> IMRHLPYFCRGQVVRGFGRGSKQLGIPTANFPEQVVDNLPADISTGIYYGWASVGSGDVHKMVVSIGWNPYYKN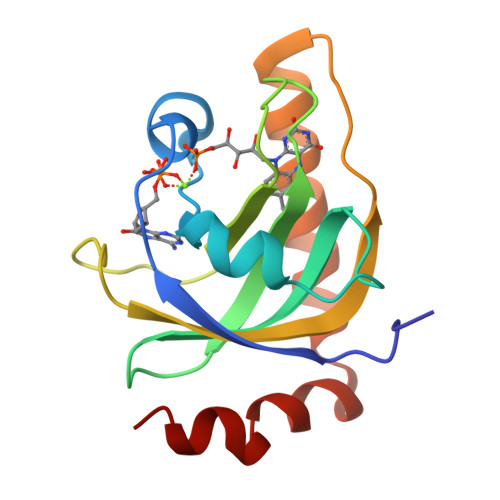TKKSMETHIMHTFKEDFYGEILNVAIVGYLRPEKNFDSLESLISAIQGDIEEAKKRLELPEYLKIKEDNFFQVSK>[2x]SNAQFGGLPVPLDQTLPLNVNPALPLSPTGLCGSLTNALSNGLLSGGLLGILENLP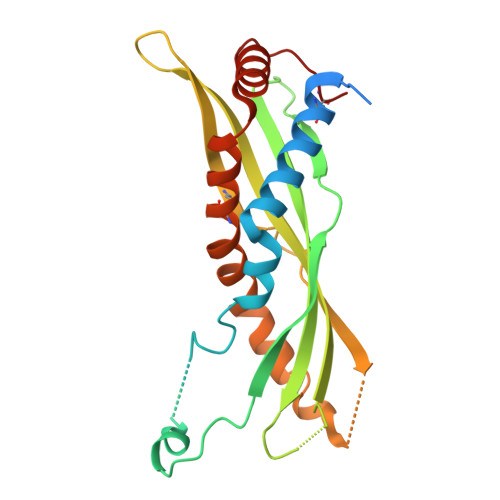LLDILKPGGGTSGGLLGGLLGKVTSVIPGLNNIIDIKVTDPQLLELGLVQSPDGHRLYVTIPLGIKLQVNTPLVGASLLRLAVKLDITAEILAVRDKQERIHLVLGDCTHSPGSLQISLLDGLGPLPIQGLLDSLTGILNKVLPELVQGNVCPLVNEVLRGLDITLVHDIVNMLIHGLQFCIKV GuaB catalyzes the oxidation of the substrate inosine-5´-monophosphate (IMP) to xanthosine 5´-monophosphate (XMP) using NAD+ as a cofactor, and guanosine 5´-monophosphate (GMP) synthase converts XMP to guanosine 5'- monophosphate (GMP) to generate guanine nucleotides essential for cell growth and viability. Indeed, genetic studies have shown that de novo guanine biosynthesis is essential for growth and viability of bacteria both in vitro and in vivo (10–23). Here, we present the first high resolution co-crystal structures of A. baumannii, S. aureus, and E. coli GuaB proteins (cystathionine beta-synthase (CBS) domains deleted), each determined with a matched set of three different inhibitors bound. Similarly, the NAD+ binding region, also where our compounds bind, occurs at the junction between neighboring molecules with side chains from both protomers contributing to ligand binding interactions.

The A. baumannii protein consistently crystallized in space group P21 with eight copies in the asu, forming an octamer composed of two inverted tetramers, relatively rotated to interdigitate the labile “finger” loops (residues 371–381) that mediate much of the tetramer:tetramer interface. We observed a tight overlay of structures across the bacterial strains, highlighting common critical interactions required for potency. These inhibitors mimic the NADH/IMP cofactor interactions by forming strong π-π stacking interactions with IMP while also hydrogen bonding with the conserved glycine (Gly299Ab/302Sa/300Ec) which is one of the two hydrogen bond interactions observed with the NADH amide. The ligand linker segment induces a 90° bend, directing either the amide N-H of G2 and G1 or the imidazole of G8 to form an important hydrogen bond to the conserved glutamic acid (Glu416Ab/417Sa/415Ec) while directing the aryl tail group into a hydrophobic shelf region. This Glu residue underpins species selectivity, because the human homologs (IMPDH1/2) contain a Gln residue at this position that effectively prevents binding. Differences in the polarity of a particular key selectivity residue specifically (Ser250 in E. coli versus Ala252 in S. aureus and Ala249 in A. baumannii) was found to be critical for inhibitor interaction with GuaB which corroborates the observations of previous reports. Enzymatic mechanism of inhibition studies showed GuaBi binds to A. baumannii GuaB uncompetitively with respect to IMP, and via a mixed non-competitive binding type with respect to NAD+. GuaBi exhibited dose-dependent bactericidal efficacy against A. baumannii in vivo. G2 was bactericidal against A. baumannii at 5× Fu/MIC, and G1 was bactericidal above 2× Fu/MIC. GuaB Y445S/N/C and A.b.GuaB P25A/S are predicted to reduce the affinity of GuaBi-binding to the enzyme based on their location in the GuaB inhibitor binding site, but further studies are required to confirm this hypothesis.

>MHHHHHHGENLYFQGSMLTIVQEALTFDDVLLLPAYSTVLPKDVSLKTRLTRGIYLNIPLVSAAMDTVTESRMAIAMAQNGGIGILHKNMDIAAQAAEVRRVKKFEAGKAESYPNSCKDDLGRLRVGAAVGTGADTPSRVEALVEAGVDVIVVDTAHGHSAGVIERVRWVKQNFPQVQVIGGNIATGDAALALLDAGADAVKVGIGPGSICTTRIVAGIGMPQISAIDSVASALKDQIPLIADGGIRFSGDMAKAIGAGASTIMVGSLLAGTEEAPGEVEFFQGRYYKAYRGMGSLGAMAGATGSADRYFQDSKAGAEKLVPEGIEGRVPYKGPMGNIVHQMMGGLRSSMGYTGSAVIEDLRQNAKFVKITSAGMSESHVHDVTITKEAPNYRVG[8x]>[2x]MGAAGDAAIGRESRELMSAANVGRTISRIAHQIIEKTALDDPVGPDAPRVVLLGIPTRGVTLANRLAGNITEYSGIHVGHGALDITLY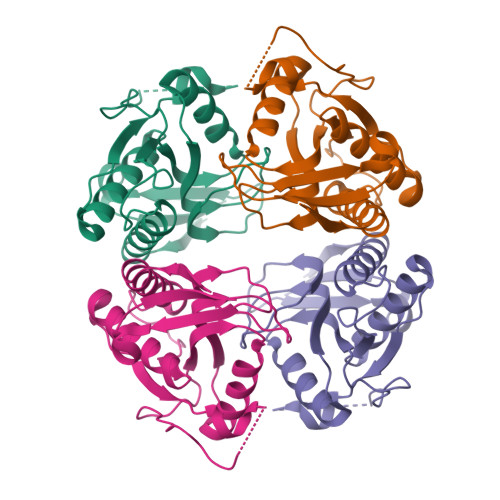RDDLMIKPPRPLASTSIPAGGIDDALVILVDDVLYSGRSVRSALDALRDVGRPRAVQLAVLVDRGHRELPLRADYVGKNVPTSRSESVHVRLREHDGRDGVVISRGSHHHHHH> MLRYTGLWRERKVEKLLVANRGEIACRVFRTCREMHIRTVALFCEAERNAKHVAEADEAVCIGPPPAVNSYL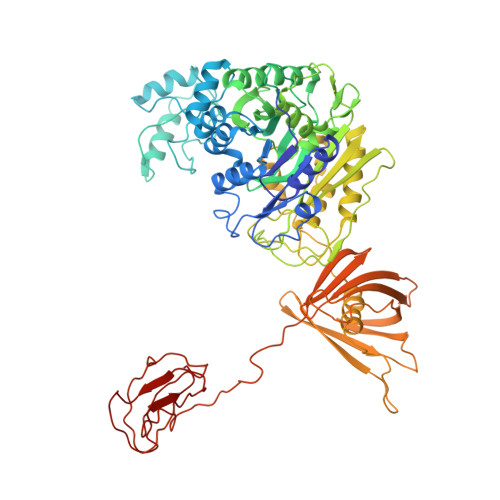RGEHIISVAKQLNVDAIHPGYGFLSENASFADAITRSGIEFIGPPASAISLMGSKSESKRIMEAAGVPVVPGYYGENQNVSFLAEEAKKVGFPILIKAVSGGGGKGMKIVERPEDFTFMLESAKREATNFFKDDRVILERYVKRSRHIECQIFFDKHGRGVFFFERDCSVQRRYQKVLEEAPAPHLSMETRQRIGEVALQAAKAVGYVGAGTVEFIFDTSTGEFYFMEMNTRLQVEHPVTEEVCRIKGAPLDLVKLQIKTAMGKPLTFSQEDVTLVGSCIEARVYAESPERGFLPESGPLTFIREPFQGVRGPARTRLDTGFREGDNVLIHYDPMLAKVISWGRSREEALRGLRQALGEYKVAGINTNIEFLKRCCETPEFARGGVTTNFISEHESQLLKSPVVTPEVAAMAATAWLLNRCDNWRGAFRLNSDTNATVHFYIDDHPVEVRLHTEGANYHKIFFSVWDHDGSFEVCSGPVTSKHRDQKSIVNDFTFLFENGMHHTVLAVATEGDVTVIGSFGLHQLRLLPLTDGFGDSSTAGGTSTKIVSPMPGKVSKLLVKSGDLVEKGQVLVIVEAMKMEHPVRALQDGRVSFLVKEGEVVGGDHVLATVAEEE> MDPIGINKVLDHLAPSELIKPVKSCHNKPSVLVLDDRIVDAATKDLYVNGFQEEIQYQNPTPENLQHMFHQGIEILDSARMINVTHLALWKPSSFKLGNPVDFALDDNYDTFWQSDGGQPHQLDIMFSKRMDICVMAIFFSMIADESYAPSLVKVYAGHSPSDARFYKMLEVRNVNGWVALRFLDNREDDQLLKCQFIRLLFPVNHENGKDTHLRGIRLYVPSNEPHQDTHEWAQTLPETNNVFQDAILR;> MTSKPSTRNDYLPRETHNGEYTGDSPEWQLQINITNKIGGINGDIWLSRDGRSVKWCIEDQCLRQFTYNQKIIKAGYIDFEKTPDCFVVVLSDIAHVYMLKNGGSTTVCFPFQIGNAFWYANGVILERETSASFMDGGYDLKPIEFDLKHKYITLTDPMAPFGLISITNTFKGGINSASGNKTDILQDFQLVLFPSDKDKCIAVFLDRNSKVLRFYYSRILSSDQSRKGELTISSTKKTGLDAAGNSQKSGGISKDLRKFSHLTRRSTSINSNSHDFNAAERVLSGNVGNASGRTDIFALPSSCSRRSLSATLDRMGNNIAPTNRAAPSGFFDSSSANTATHSNITPVSQPMQQQQQEYLNQTATSSKDIVLTEISSLKLPDDIIFTSRRLSSILSKLKFLSLRFERREGLLIFHEPTHFCKIWLIDLLPDVLDSIPFKIYGNSPQNMIRLENLKLKEPSRIQAMYIHELLESCLILVSEGQNKEEYKACLYDPFVKITSPSKNISEELTKQNSLPSLQKLFPYPETSFTKLCFEAVKYITSPAFNISFIFLWQSAYSILLSRANDDVVGGLKMEHDAFSLVLSLLILPIPSSSAQEYQEYKEIYERDLFQHLKQDSEITSSVLPRIVIGLHLIREEYSLNVLCRNEHALLGQFLRFATAAMGWPDLWQSYYVPKMDSESKTFLHPREQNSTFFHPLDEPPSITKSLYSITENSSIPLCPFISFSRLVATDTQVELRITPRSFKILGLYELVHSPNFLPDYVLGILSSFKVDKDELQTYPLGILVPLQNILKILEDKLSEVRDNLELLDRADLQRCSAIINSIRSDSKEVLKRGQRDSYMLCKVPLAKNRSSLSKKPSDIYSILSEIVKSASQVPLDGSAMRMSNIQDDEDIDEGRSLKLNAGLIFSEDKRFTHVVSLLAYYRPTKTQFFTTKTEYAQILAQKKYFAKIMALRTCTNGVGWGAVAYATEKPISTQKWVIQPLNLISVFPDDTKITVKAPEDIAHDIVEWGQFHAGVSSGLRISKKATGIT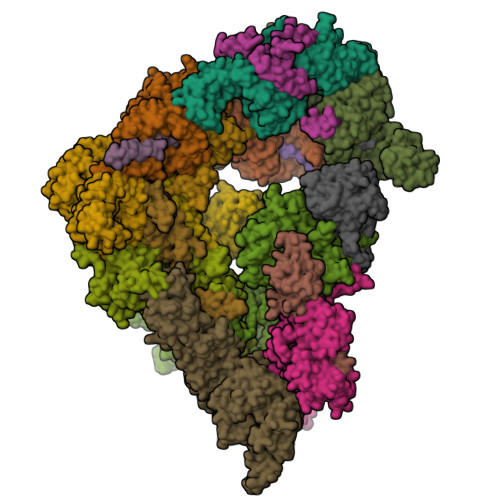GSWIAFNKPKELDAYHGGFLLGLGLNGHLKNLEEWHIYNYLSPRNTHISIGLLLGMSSSMKGSMDSKLIKVISVHLVAFLPSGSSDLNIDLKLQTAGIIGMGMLYLNSRHKRMSDSIFAQLVSLLNVNDEMVADEEYRLAAGISLGLINLGAGQTKLRKWDSSLLGLGDDLPEDVYDSSDVEQNVMYEDLTTKLLEIVTSTYDVENDWIPENSQIGAVIAIMFLFLKSNNFGISNMLKVDLKEILKANINTRPELLMYREWASNMILWEFIGDDLSFIMKDVDIGVKFSELNTDLLPIYYTMAGRILAMGIRFASTGNLKIRNILLSLVDKFLPLYQYPGKQNLDFRLTISVINVLTNVIVVSLSMVMCASGDLEVLRRVKYLHEVASGPYSDLFQEIPSSKSDVSGVTQVTSNTNTPGNSDRERVDETAASLDDERSSNGSDISDPTAYLEDKKDIDDHYGKFISTNLALGFLFLGSGQYALNTSTLESIAFLSMSVLPTYTTPHPLQELKHFWSMAVEPRCLVIKDISTGDAVNNVPIELVVEEDVEKEEVIREISTPCLLPDFSKIKSIRVKMHGYFPLEVNFTKDYSASDFFSGGTIIYIQRKSESVFENKASFRNVEDIHVALKRKAAESKNYSRLNLKNEQGNTTSSQLVESLGIQDLTMVELDTLLSAGNNTALTDSESYNLGLLCSDKNSGDILDCQLELWYKSFGPHDE;>[2x]MNDDSQDKIIHDIRIQLRKAATELSRWKLYGSSKWAAEALAGLAEAIDVDQTHSLADESPLRNKQGVPKQMFEIPQNGFGLSETEYDLYLLGSTLFDAKEFDRCVFFLKDVTNPYLKFLKLYSKFLSWDKKSQESMENILTTGKFTDEMYRANKDGDGSGNEDINQSGHQRANLKMVSNEHESQSNISSILKEINTFLESYEIKIDDDEADLGLALLYYLRGVILKQEKNISKAMSSFLKSLSCYSFNWSCWLELMDCLQKVDDALLLNNYLYQNFQFKFSENLGSQRTIEFNIMIKFFKLKVFEELNGQLEDYFEDLEFLLQVFPNFTFLKAYNATISYNNLDYVTAESRFDDIVKQDPYRLNDLETYSNILYVMQKNSKLAYLAQFVSQIDRFRPETCCIIANYYSARQEHEKSIMYFRRALTLDKKTTNAWTLMGHEFVELSNSHAAIECYRRAVDICPRDFKAWFGLGQAYALLDMHLYSLYYFQKACTLKPWDRRIWQVLGECYSKTGNKVEAIKCYKRSIKASQTVDQNTSIYYRLAQLYEELEDLQECKKFMMKCVDVEELLEGIVTDETVKARLWLAIFEIKAGNYQLAYDYAMGVSSGTSQEIEEARMLARECRRHM;> MNQNGDKNEGKLFQLPSLPPWKTPRFNKANFNNFTTPLRKRSTRVINDDSMPITGEVLEERTADDLYGINMDVDEVDYLNTLSHIEEEKQYDYSPFCERNTLRESRIDSFLKAERAAHCLVFHKVGHLDGIDSYRPDIDIMCGEEANKYDSANPEGNGSMLLESVPGCNKEDLERLSRREFVTNSKPNMRRLDDIINHETNALKSFWNDSGLVNSLQSHHLHEEYLLLQEELKNVYKIKCHDRVPIESLRDKCRRHYSNEDSSFL;>[2x]MAVNPELAPFTLSRGIPSFDDQALSTIIQLQDCIQQAIQQLNYSTAEFLAELLYAECSILDKSSVYWSDAVYLYALSLFLNKSYHTAFQISKEFKEYHLGIAYIFGRCALQLSQGVNEAILTLLSIINVFSSNSSNTRINMVLNSNLVHIPDLATLNCLLGNLYMKLDHSKEGAFYHSEALAINPYLWESYEAICKMRATVDLKRVFFDIAGKKSNSHNNNAASSFPSTSLSHFEPRSQPSLYSKTNKNGNNNINNNVNTLFQSSNSPPSTSASSFSSIQHFSRSQQQQANTSIRTCQNKNTQTPKNPAINSKTSSALPNNISMNLVSPSSKQPTISSLAKVYNRNKLLTTPPSKLLNNDRNHQNNNNNNNNNNNNNNNNNNNNNNNNIINKTTFKTPRNLYSSTGRLTTSKKNPRSLIISNSILTSDYSITLPEIMYNFALILRSSSQYNSFKAIRLFESQIPSHIKDTMPWCLVQLGKLHFEIINYDMSLKYFNRLKDLQPARVKDMEIFSTLLWHLHDKVKSSNLANGLMDTMPNKPETWCCIGNLLSLQKDHDAAIKAFEKATQLDPNFAYAYTLQGHEHSSNDSSDSAKTCYRKALACDPQHYNAYYGLGTSAMKLGQYEEALLYFEKARSINPVNVVLICCCGGSLEKLGYKEKALQYYELACHLQPTSSLSKYKMGQLLYSMTRYNVALQTFEELVKLVPDDATAHYLLGQTYRIVGRKKDAIKELTVAMNLDPKGNQVIIDELQKCHMQE;>MIRRAPTTLQLSHDDVTSLIDDLNEQKLKQQLNIEKTKYFQGKNGGSLHSNTDFQDTSQNIEDNNNDNDNDIDEDDDMSSYNDKAASVAHTRVLNSLHLSTDSNTAHETSNANDNHNPFYIREE[2x];> MSSSSYRDSYFQYRHLPAPHHILYAEWNQDILALPDEVANITMAMKDNTRTDAEEGRAPQDGERNSNVRESAQGKALMTSEQNSNRYWNSFHDEDDWNLFNGMELESNGVVTFAGQAFDHSLNGGTNSRNDGANEPRKETITGSIFDRRITQLAYARNNGWHELALPQSR;>[2x]MKFCLYCCHCYIVICGKATHYYKSSKATSNLKSSNRVLMRNPMSPSEQHSQHNSTLAASPFVSNVSAARTQQSLPTDAQNDRLQQPWNRTNTATSPYQSLANSPLIQKLQANIMTPHQPSANSNSNSNSITGNVVNDNNLLASMSKNSMFGSTIPSTLRKVSLQREYKDSVDGVVRDEDNDEDVHNNGDAAANANNDRESKLGHNGPLTTTTLTTTTTATQLDVSELSAIERLRLWRFDALMQHMYRTAEYIADKVYNISNDPDDAFWLGQVYYNNNQYVRAVELITRNNLDGVNILCRYLLGLSFVKLQRFDDALDVIGEYNPFSEDPSTTAANTMSNNGNNSNTSQPVTDGGIKMESSLCFLRGKIYFAQNNFNKARDAFREAILVDIKNFEAFEMLLSKNLLTPQEEWDLFDSLDFKEFGEDKEIMKNLYKINLSKYINTEDITKSNEILAKDYKLADNVDVVRSKVDICYTQCKFNECLELCETVLENDEFNTNILPAYIGCLYELSNKNKLFLLSHRLAETFPKSAITWFSVATYYMSLDRISEAQKYYSKSSILDPSFAAAWLGFAHTYALEGEQDQALTAYSTASRFFPGMHLPKLFLGMQFMAMNSLNLAESYFVLAYDICPNDPLVLNEMGVMYFKKNEFVKAKKYLKKALEVVKDLDPSSRTTISIQLNLGHTYRKLNENEIAIKCFRCVLEKNDKNSEIHCSLGYLYLKTKKLQKAIDHLHKSLYLKPNNSSATALLKNALELNVTLSLDASHPLIDKSNLMSQASKDKASLNKKRSSLTYDPVNMAKRLRTQKEIFDQNNKALRKGGHDSKTGSNNADDDFDADMELEKSSIPENLYF;> MARALRDISLFNDIRKDQNSAGAKHERYNMRDLRSKKNQHVNGIDDYEDDSLDRFIRRKKSRVVKYIPSLSAYNVFNEFPYYPTSASQLLDGKLDEFLMLSEQYKSRLPKIRKLGWNRFKPIGINKTMYELEMLRSRARAQNAEGNNEEDFRQHDSREEDPRNNGSIGRVILPHILQENEEYDTGEGVTGLHSMPNDSMAILANNSANNSQNEEVSEEDEISYDYDAEFDHVVDEDDNEEGEVPGEGVEGIEVQRERIVPDDLLMRPTSLSRSLQQFVEEAHHLDRNPYDIDSDNDGEDSKVELDMNPDFEDDVGREHDYNSEYSQEPTSYGGITPDLASNWRNWTRERITSLDELMERRARQQRGQD;> MSKYGPLGITNFITPYDLCILILIHAHCSQDNGISVPTAVFLRLISPTRPSLEWNPLLKDNSNLRSSSIVPPPVLPILDNIIRILLDDKDGNKIALTLMGYLEAINGLDSINRLMMDLEKNCLVNNYRSMKMRTTSTRRQMTRASFLGTFLSTCIRKYQIGDFEMRETIWINLQNFKTVFKHTPLWLRFKDNVHIQKVKNCLLANDEISVEDQQMVEFFQHFNNGNDADSKTMNEENYGTLISIQHLQSIVNRQIVNWLDNTEFNLMGQEETSSTYEEQSGLVFDLLDTLSLNDATKFPLIFILKYLEAIKENSYQTALDSLHNYFDYKSTGNSQNYFHISLLSLATFHSSFNECDAAINSFEEATRIARENKDMETLNLIMIWIINFIEVHPEYANRFYITVEQIIKYLKNSSDVEDANIFSNAYKFETLLSMVKESKTAEVSSSLLKFMAITLQNVPSQNFDLFQSLVSYEVKFWKELGYESISDVYEKFLSKTSSSSLRNYDSSIINQDIKVAFKALEEDDFLKVKQYLLKSESLELDYDQKINLKYLRVKYLVKIGDYDLSMRLINQYVKECCEEVADSNWRFKFEIESINVLLLSDVGIRSLPKIIKLIDEYKEIGNPLRCVILLLKLCEVLIQVGKSMEAECLISCNLSTILEFPFVRKKTDELLESLSVEEDRDVQMT;> MSSPINDYFIDYNPLFPIFATRIAKGLAIYRVSDHARLAVIPIRNINLVANYDWDTTTGKFLSIFFKDGTIRIHDIFKDGRLVSFLRIPSTKISKGIWDRIPLRYEPNNRDFACNIIDDLPKLIRFVKDSKRINIVPYTQPNSLWRGPDEDDLDSNEKLDVHVVFNEGNDKITVFFNGDYAVFLSVDNIENENSLKSIIKVQDGFYQCFYEDGTVQTLNLGPLLQSKSSVNLLNYIMVIKELIGYMLTHLEFINRELATPYLDFVKRLCDEAYGYGKLKSELEALFLLGEISCDLEDWLCNSVGEKNFKRWKYLGCEAYQKTVQILTLIFVPACERIIIYVEKLRAILQAFSIQNKLSYTSDLTAVEVLLKSSQKLLTMTLNSIIGLGRDETLFEKFFIWFNDRLHEALDEDYKLKFQFEDDLYFGYDLLSYFDRILSKKGTEPSSIIDVKLYRDLINSMSDMEKDIAQSNVNSHIQQHILVDLKTDVFAQKYPSSQINLLDAIKLPKHNYIVYLIQVTKHNSAQEPFSEENKKKLYIGTLKDENLGIISKESSVKIPALFKSYRLSSTRFVPNRVHSLLRDIGLSDSNYHSSHVTDYRGENYENEEDDGTIAIPAYIRENRENDDFIACTAKVSVDGRSASLVFPKEKQNV;> MSFQITPTRDLKVITDELQTLSSYIFHTNIVDDLNSLLTWMSPNDAKSNHQLRPPSLRIKNIIKVLFPNNATTSPYSMINTSQANNSIVNEGNTNKELQLQLFSTLKEFYIFQVRYHFFLHFNNINYLKDIQRWENYYEFPLRYVPIFDVNVNDWALELNSLRHYLLNRNIKFKNNLRTRLDKLIMDDDFDLADNLIQWLKSANGSLSSTELIVNALYSKINKFCEDNMSRVWNKRFMIMETFNKFINQYWSQFSKLVGCPEDDHELTTTVFNCFESNFLRIRTNEIFDICVLAYPDSKVTLLELRKIMKDFKDYTNIVTTFLSDFKKYILNPSVTTVDALLRYVKTIKAFLVLDPTGRCLHSITTFVKPYFQERKHLVNVLLYAMLDLPEEELKEKINFNVDMKALLSLVDTLHDSDINQDTNITKRDKNKKSPFLWNLKVKGKRELNKDLPIRHAMLYEHILNYYIAWVPEPNDMIPGNIKSSYIKTNLFEVLLDLFESREFFISEFRNLLTDRLFTLKFYTLDEKWTRCLKLIREKIVKFTETSHSNYITNGILGLLETTAPAADADQSNLNSIDVMLWDIKCSEELCRKMHEVAGLDPIIFPKFISLLYWKYNCDTQGSNDLAFHLPIDLERELQKYSDIYSQLKPGRKLQLCKDKGKVEIQLAFKDGRKLVLDVSLEQCSVINQFDSPNDEPICLSLEQLSESLNIAPPRLTHLLDFWIQKGVLLKENGTYSVIEHSEMDFDQAQKTAPMEIENSNYELHNDSEIERKYELTLQRSLPFIEGMLTNLGAMKLHKIHSFLKITVPKDWGYNRITLQQLEGYLNTLADEGRLKYIANGSYEIVKNGHKNS;> MKVKINEVHSVFAWSWHIPSTSDEDAANNDPIGNDEDEDVCGICRASYNGTCPSCKFPGDQCPLVIGLCHHNFHDHCIYRWLDTPTSKGLCPMCRQTFQLQKGLAINDAHVQKFVEIVSRRREEMIEEGVAEEFVDFDEPIRQNTDNPIGRQQVDTILDEDFLLR> GQQGLAEVAVRLQEPIVLGPRTLQVSWTVDGPVQLVQGFRVSWRVAGPEGGSWTMLDLQSPSQQSTVLRGLPPGTQIQIKVQAQGQEGLGAESLSVTRSIPEEAPSGPPQGVAVALGGDGNSSITVSWEPPLPSQQNGVITEYQIWCLGNESRFHLNRSAAGWARSAM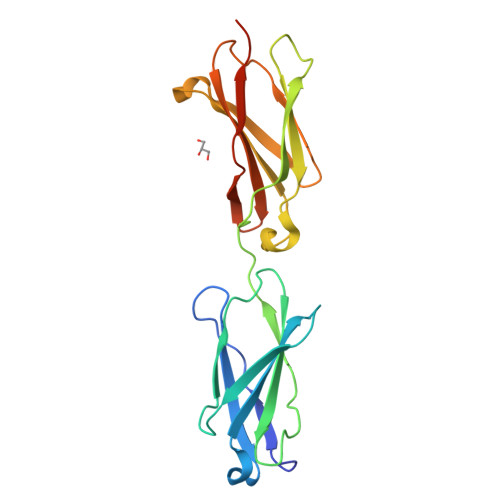LRGLVPGLLYRTLVAAATSAGVGVPSAPVLVQLPSPPDLHHHHHH XANTHINE | C5 H4 N4 O2 | 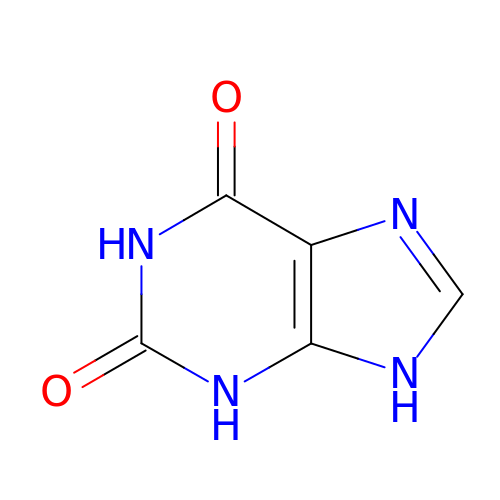LRFVTYWOQMYALW-UHFFFAOYSA-N2-[(2,6-dichloro-3-methyl-phenyl)amino]benzoic acid | C14 H11 Cl2 N O2 | 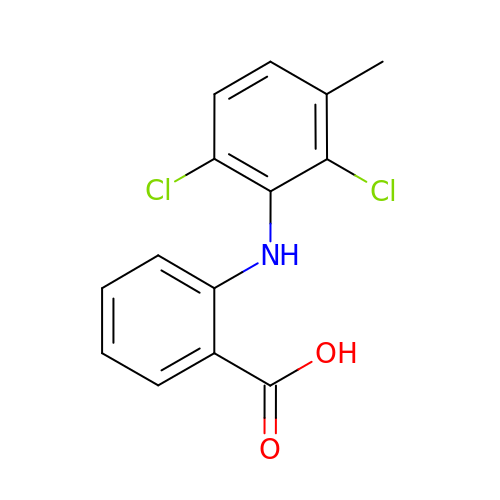SBDNJUWAMKYJOX-UHFFFAOYSA-N>MGAASDQHRSRRHDESSSRPNKKKKVSRNPETNLLFNLNSCSKSKDLSAALALYDAAITSSEVRLSQQHFQTLLY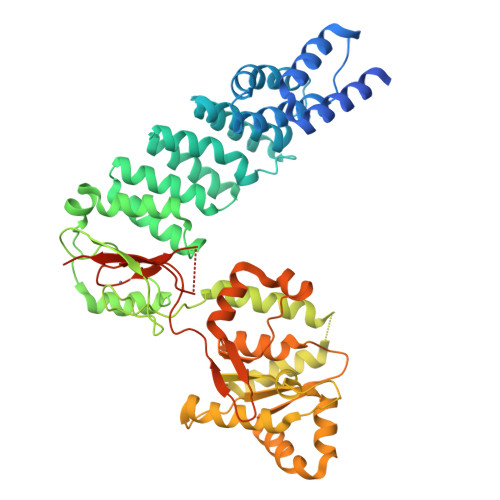LCSASITDISLQYLAIDRGFEIFDRMVSSGISPNEASVTSVARLAAAKGNGDYAFKVVKEFVSVGGVSIPRLRTYAPALLCFCEKLEAEKGYEVEEHMEAAGIALEEAEISALLKVSAATGRENKVYRYLHKLREYVGCVSEETLKIIEEWFCGEKAGEVGDNGIGSDVGMLREAVLNNGGGWHGHGWVGEGKWTVKKGNVSSTGRCLSCSEQLACVDTNEVETQKFVDSLVALAMDRKTKMNSCETNVVFSEFQDWLEKHGDYEAIVDGANIGLYQQNFVDGSFSLSQLESVMKELYRESGNNKWPLILLHKRRVKTLLENPTHRNLVEEWISNGVLYATPPGSNDDWYWLYAAAKLKCLLVTNDEMRDHIFELLGSTFFQKWKERHQVRYTFVKGNLKLEMPSPFSVVIQESEKGSWHFPVSCENNEESSRTWMCISRQSILDSPKSNGKIPLEHHHHHH[2x]> MAIELNVGRKVTVTVPGSSANLGPGFDTLGLALSVYDTVEVEIIPSGL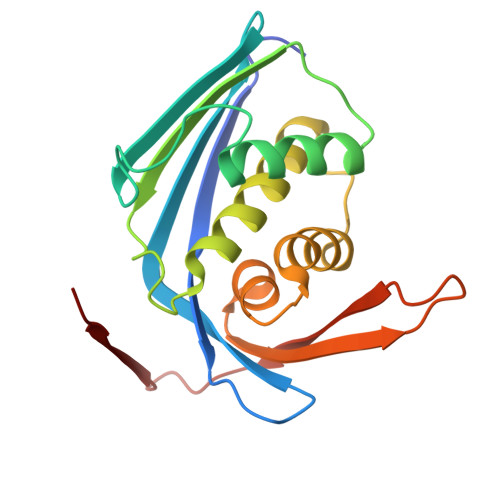EVEVFGEGQGEVPLDGSHLVVKAIRAGLKAADAEVPGLRVVCHNNIPQSRGLGSSAAAAVAGVAAANGLADFPLTQEQIVQLSSAFEGHPDNAAASVLGGAVVSWTNLSIDGKSQPQYAAVPLEVQDNIRATALVPN>[2x]MLDYFFNPKGIAVIGASNDPKKLGYEVFKNLKEYKKGKVYPVNIKEEEVQGVKAYKSVKDIPDEIDLAIIVVPKRFVKDTLIQCGEKGVKGVVIITAGFGETGEEGKREEKELVEIAHKYGMRIIGPNCVGIMNTHVDLNATFIT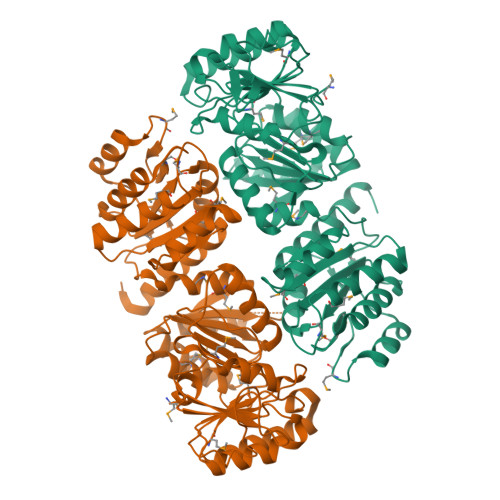VAKKGNVAFISQSGALGAGIVYKTIKEDIGFSKFISVGNMADVDFAELMEYLADTEEDKAIALYIEGVRNGKKFMEVAKRVTKKKPIIALKAGKSESGARAASSHTGSLAGSWKIYEAAFKQSGVLVANTIDEMLSMARAFSQPLPRGNKVAIMTNAGGPGVLTADELDKRGLKLATLEEKTIEELRSFLPPMAAVKNPVDMIASARGEDYYRTAKLLLQDPNVDMLIAICVVPTFAGMTLTEHAEGIIRAVKEVNNEKPVLAMFMAGYVSEKAKELLEKNGIPTYERPEDVASAAYALVEQAKNVGILEVE> GIDPFTMATFISVQLKKTSEVDLAKPLVKFIQQTYPSGGEEQAQYCRAAEELSKLRRAAVGRPLDKHEGALETLLRYYDQICSIEPKFPFSENQICLTFTWKDAFDKGSLFGGSVKLALASLGYEKSCVLFNCAALASQIAAEQNLDNDEGLKIAAKHYQFASGAFLHIKETVLSALSREPTVDISPDTVGTLSLIMLAQAQEVFFLKATRDKMKDAIIAKLANQAADYFGDAFKQCQYKDTLPKEVFPVLAAKHCIMQANAEYHQSILAKQQYYFGEEIARLQHA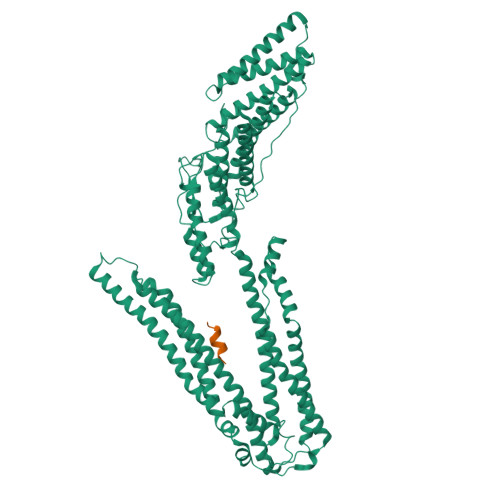AELIKTVASRYDEYVNVKDFSDKINRALAAAKKDNDFIYHDRVPDLKDLDPIGKATLVKSTPVNVPISQKFTDLFEKMVPVSVQQSLAAYNQRKADLVNRSIAQMREATTLANGVLASLNLPAAIEDVSGDTVPQSILTKSRSVIEQGGIQTVDQLIKELPELLQRNREILDESLRLLDEEEATDNDLRAKFKERWQRTPSNELYKPLRAEGTNFRTVLDKAVQADGQVKECYQSHRDTIVLLCKPEPELNAAIPSANPAKTMQGSEVVNVLKSLLSNLDEVKKEREGLENDLKSVNFDMTSKFLTALAQDGVINEEALSVTELDRVYGGLTTKVQESLKKQEGLLKNIQVSHQEFSKMKQSNNEANLREEVLKNLATAYDNFVELVANLKEGTKFYNELTEILVRFQNKCSDIVFAR;> AAGAYDPARKLLEQYAKK> MQSQAISNYENKVEKLDTSKADEMRAAAEVYNQTLEKGVVPNYRLSEEEKRTYNSLLDVTGTGIMAYVEIPKLGTNLPIYHGTDDAILQVAIGHIPGSSL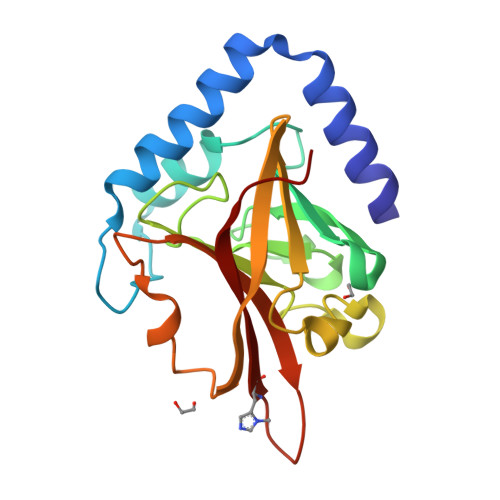PVGGQGTHSVISGHRGLPSAKLFTDIDKLKNGDRFMIHVLGKTITYQVDQTLTVEPEDISSLAIDPDQDYCTLVTATPYGINSHRLLVRGHRVPNEK> MILDVDYITEEGKPVIRLFKKENGKFKIEHDRTFRPYIYALLRDDSKIEEVKKITGERHGK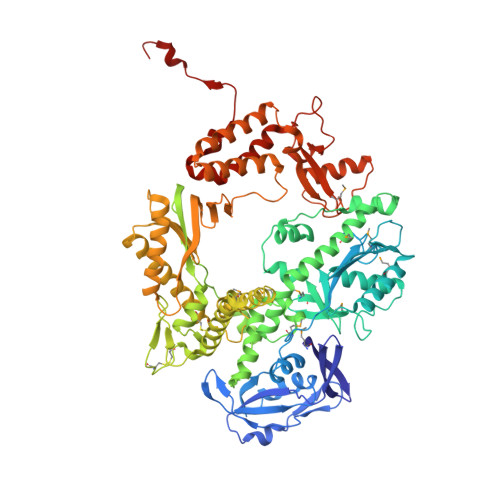IVRIVDVEKVEKKFLGKPITVWKLYLEHPQDVPTIREKVREHPAVVDIFEYDIPFAKRYLIDKGLIPMEGEEELKILAFDIETLYHEGEEFGKGPIIMISYADENEAKVITWKNIDLPYVEVVSSEREMIKRFLRIIREKDPDIIVTYNGDSFDFPYLAKRAEKLGIKLTIGRDGSEPKMQRIGDMTAVEVKGRIHFDLYHVITRTINLPTYTLEAVYEAIFGKPKEKVYADEIAKAWESGENLERVAKYSMEDAKATYELGKEFLPMEIQLSRLVGQPLWDVSRSSTGNLVEWFLLRKAYERNEVAPNKPSEEEYQRRLRESYTGGFVKEPEKGLWENIVYLDFRALYPSIIITHNVSPDTLNLEGCKNYDIAPQVGHKFCKDIPGFIPSLLGHLLEERQKIKTKMKETQDPIEKILLDYRQKAIKLLANSFYGYYGYAKARWYCKECAESVTAWGRKYIELVWKELEEKFGFKVLYIDTDGLYATIPGGESEEIKKKALEFVKYINSKLPGLLELEYEGFYKRGFFVTKKRYAVIDEEGKVITRGLEIVRRDWSEIAKETQARVLETILKHGDVEEAVRIVKEVIQKLANYEIPPEKLAIYEQITRPLHEYKAIGPHVAVAKKLAAKGVKIKPGMVIGYIVLRGDGPISNRAILAEEYDPKKHKYDAEYYIENQVLPAVLRILEGFGYRKEDLRYQKTRQVGLTSWLNIKKS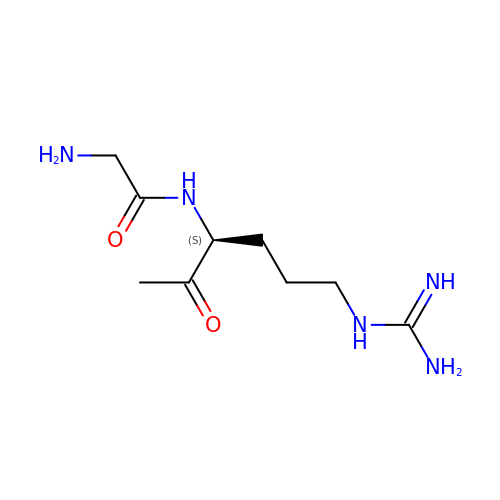N-[(3S)-6-carbamimidamido-2-oxohexan-3-yl]glycinamide | C9 H19 N5 O2 | CAKKYWQZWULXCC-ZETCQYMHSA-N5'-O-MONOPHOSPHORYLADENYLYL(2'->5')ADENYLYL(2'->5')ADENOSINE | C30 H38 N15 O19 P3 | 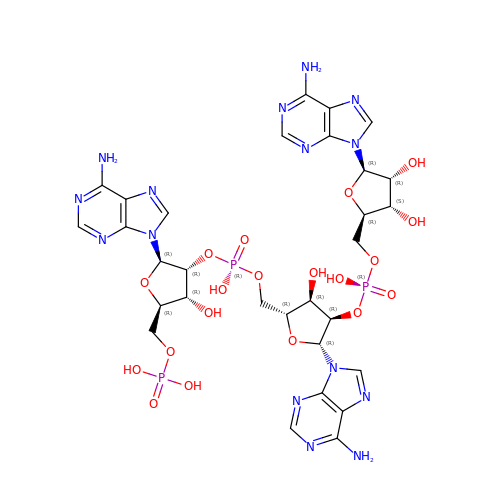SIIZPVYVXNXXQG-UQTMIEBXSA-N>[5x]PLIRIDLT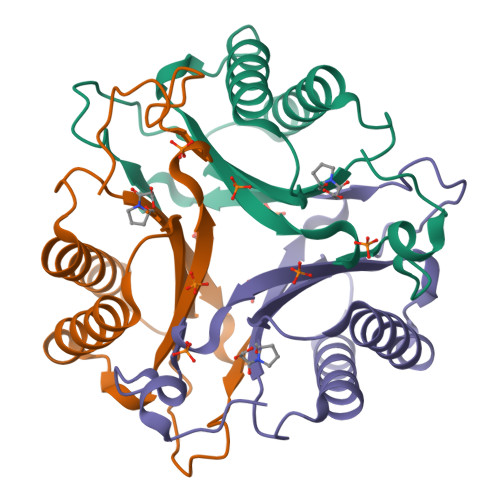SDRSREQRRAIADAVHDALVEVLAIPARDRFQILTAHDPSDIIAEDAGLGFQRSPSVVIIHVFTQAGRTIETKQRVFAAITESLAPIGVAGSDVFIAITENAPHDWSFGFGSAQYVTGELAIPATGAA~{N}-[2-methyl-3-(3-methyl-4-oxidanylidene-5,6,7,8-tetrahydro-2~{H}-cyclohepta[c]pyrrol-1-yl)phenyl]methanesulfonamide 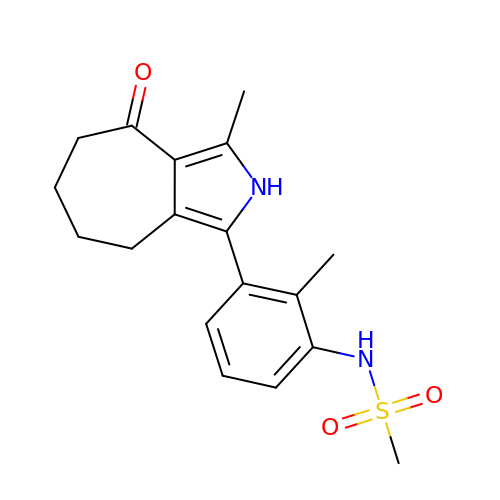| C18 H22 N2 O3 S | VUJHBAXRQCRYLD-UHFFFAOYSA-N>YKWHYSGLNRWHGAGSTADFQKIIQERCDTYTQTIRPGSRSRNCQAIRQAFMSAFISKDPCKATKEDYNSLINLAPPTVPCGQQVFWSKTKELAHEYAKRRRLMTLEDTLLGYLADGLRWCGEPGSSDLNIWSCPDWRKDCRTNYLSVFWEVLSERFAESA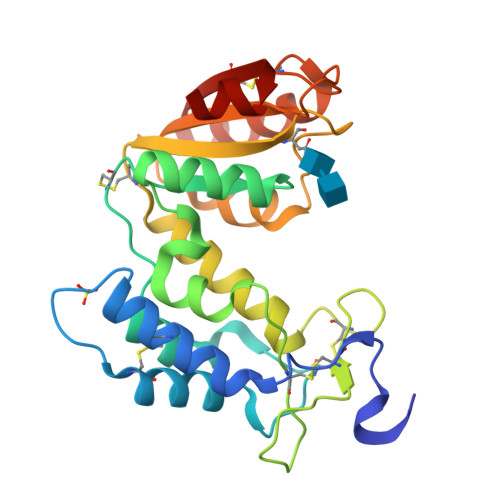CNTVRVVLNGSLENAFDSMSIFGRVEAPNLRPQVELEAWLVHDTGKPPSDSCSGSSIRKLKSILDGRNVKFRCMDNLSRDQFLQRS[2x]pmcAlcohol dehydrogenases (ADHs EC 1.1.1.1) are NAD(P)H‐dependent medium‐chain oxidoreductases found in all kingdoms of life. These enzymes typically catalyse the reversible reduction of aldehydes or ketones to the corresponding alcohol. The structural motifs of ADHs are highly conserved in all known eukaryotic examples; most notably, a zinc ion involved in catalysis, a second zinc ion involved in maintaining protein structure, and the Rossmann peptide‐fold involved in cofactor binding. ADHs have been shown to catalyse many complex biochemical transformations in plant natural product biosynthesis, suggesting that their catalytic repertoire has been expanded.

Here we report the crystal structure of dihydroprecondylocarpine acetate synthase (DPAS), an ADH that catalyses the non‐canonical 1,4‐reduction of an α,β‐unsaturated iminium moiety. We report four crystal structures of apo‐ and substrate‐bound DPAS from two phylogenetically related species. These structures reveal, surprisingly, the loss of the catalytic zinc ion from the DPAS active site, indicating that zinc is not strictly required for reduction by ADHs. Despite the presence of NADP+ in DPAS crystallisation conditions, none of the solved structures had sufficient density to model the cofactor. Therefore, to assess the position of the bound substrate relative to the cofactor, NADPH was docked into the active site of DPAS co‐crystallised with the substrate precondylocarpine acetate. The 4‐pro‐R hydride of NADPH was measured to be 3.7 Å from C19 of the substrate which is consistent with hydride addition at this carbon. Additionally, the 4‐pro‐R hydride was 4.6 Å from C15, which is the site of the second reduction to form secodine, although we note that dehydrosecodine may bind in a different orientation within the substrate cavity. Although electron density for the structural zinc ion was clearly observed in all TiDPAS2 structures (the CrDPAS structure lacked electron density for this region), surprisingly, the substrate pocket lacked electron density at the expected site of the catalytic zinc. The lack of the catalytic zinc in DPAS is substantiated by the observation that two of the conserved catalytic zinc coordinating residues are mutated (His74Met and Cys168Ser). Computational estimation found TiDPAS2 had a larger substrate cavity than other structures of ADHs involved in monoterpene indole alkaloid (MIA) biosynthesis.

>[2x]MAGKSPEEEHPVKAYGWAVKDRTTGILSPFKFSRRATGDNDIRIKILYCGICHTDLTSVKNEYEFLSYPLVPGMEIVGIATEVGSKVTKIKVGEKVAVAAYLGTCGKCYNCVNDLENYCPEVIIGYGTPYHDGTINYGGLSNETVVNERFVLRFPEKLSPAGGAPLLSAGITAYSAMRNHGLDKPGIHLGVVGLGGLGHLAVKFAKAFGVRVTVISTTPSKKDEAINNLGADAFLFSRDDKQMRAAIGTFDAIIDTLAVVHPIAPLLDLLRSHGKLVLVGAPSKPLELPTIPLLSGGKSLIGSAAGNVKQTQEMLDFAAEHDITANIEVIPIDYINTAMERLDKGDIRFRFVVDIENTLTPPPEP> TVAYIAIGSNLASPLEQVNAALKALGDIPESHILTVSSFYRTPPLGPQDQPDYLNAAVALETSLAPEELLNHTQRIELQQGRVRKAERWGPATLDLDIMLFGNEVINT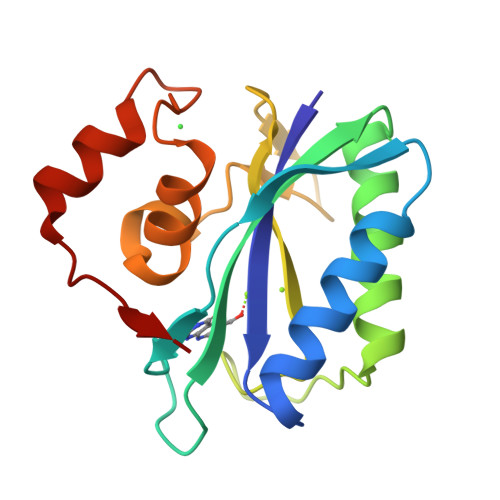ERLTVPHYDMKNRGFMLWPLFEIAPELVFPDGEMLRQILHTRAFDKLNKW pentane-2,4-dione | C5 H8 O2 | 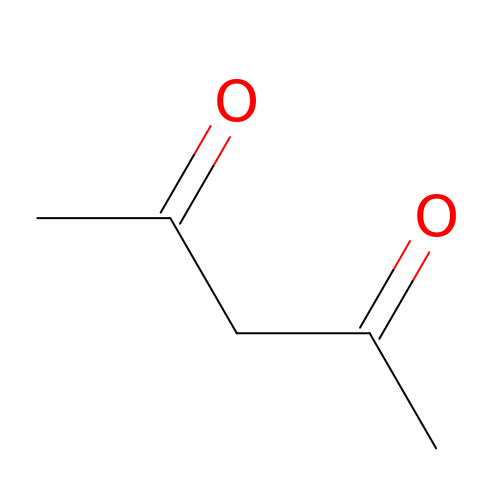YRKCREAYFQTBPV-UHFFFAOYSA-N> MHHHHHHASENLAFQGAMASSIDISKINSWNKEFQSDLTHQLATTVLKNYNADDALLNKTRLQKQDNRVFNTVVSTDSTPVTNQKSSGRAWLFAATNQLRLNV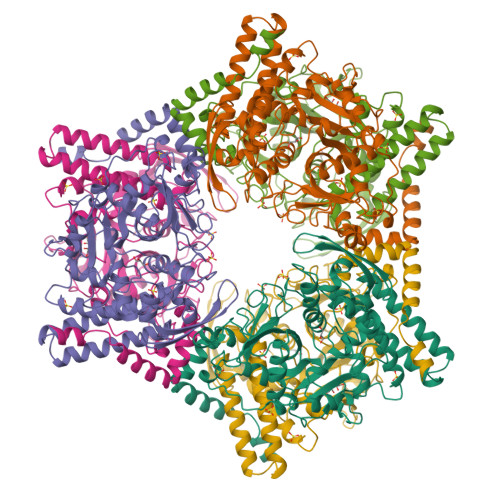LSELNLKEFELSQAYLFFYDKLEKANYFLDQIVSSADQDIDSRLVQYLLAAPTEDGGQYSMFLNLVKKYGLIPKDLYGDLPYSTTASRKWNSLLTTKLREFAETLRTALKERSADDSIIVTLREQMQREIFRLMSLFMDIPPVQPNEQFTWEYVDKDKKIHTIKSTPLEFASKYAKLDPSTPVSLINDPRHPYGKLIKIDRLGNVLGGDAVIYLNVDNETLSKLVVKRLQNNKAVFFGSHTPKFMDKKTGVMDIELWNYPAIGYNLPQQKASRIRYHESLMTHAMLITGCHVDETSKLPLRYRVENSWGKDSGKDGLYVMTQKYFEEYCFQIVVDINELPKELASKFTSGKEEPIVLPIWDPMGALA Glycan uptake across the bacterial outer membrane (OM) of these bacteria is mediated by SusCD protein complexes, comprising a membrane-embedded barrel and a lipoprotein lid, that is thought to open and close to facilitate substrate binding and transport. Here we show that for both the levan and dextran utilisation systems of Bacteroides thetaiotaomicron, the additional OM components assemble on the core SusCD transporter, forming stable glycan utilising machines which we term ‘utilisomes’. Transport-competent FOS are generated from levan by a surface-exposed lipoprotein, a GH32-family levan endo-glycanase (GHlev), while an SGBP (SGBPlev) is thought to recruit levan at the cell surface. Single particle cryogenic electron microscopy (cryoEM) structures in the absence and presence of substrate reveal concerted conformational changes that demonstrate the mechanism of substrate capture, and rationalise the role of each component in the utilisome.

The density is compatible with ~12 β2,6-linked fructose units in an extended conformation, with a putative β2,1 decoration on Frc-7. Levan binding at this tethering site is also seen in GHlev in the absence of bridging interactions with SGBPlev and in crystal structures of the inactive levanase solved in the presence of FOS of DP ~7-8 (ED Fig. 8). Indeed, secondary binding sites are relatively common in endo-acting GH enzymes, where they may enhance substrate processivity. No ligand was observed at the secondary site in a GHlev structure complexed to a 4 unit FOS (PDB ID 6R3U28), suggesting the affinity for short FOS is low. Single substitution of aromatic residues (to alanine) near the GHlev active site (Y70A and W318A) decreased affinity for levan 25-30 fold, while equivalent substitutions at the tethering site FOS4 had a 6-fold decrease in affinity (W217A) or no effect (F243A and Y437A). These results suggest the active site (FOS3) is responsible for most of the affinity of GHlev for levan. However, numerous weak interactions within the extensive secondary site (FOS4) including polar residues, may result in a substantial overall affinity and specificity.

>[2x]MMKNMILPIAFTALIASMTACSDETDPILTQKNWDGTATYFQSSDEHGFSMYYKPQVGFVGNPMPFYDPVAKDFKVMYLQDYRPNPEATYHPIFGVATKDGATYESLGELISCGGRDEQDAAIGTGGTIYNPADKLYYTFYTGNKFKPSSDQNAQVVMVATSPDFKTWTKNRTFYLKGDTYGYDKNDFRDPFLFQTEDGVYHMLIATRKNGKGHIAEFTSADLKEWESAGTFMTMMWDRFYECPDVFKMGDWWYLIYSEQASFMRKVQYFKGRTLEDLKATTANDAGIWPDNREGMLDSRAFYAGKTASDGTNRYIWGWCPTRAGNDNGNVGDVEPEWAGNLVAQRLIQHEDGTLTLGVPDAIDRKYTSAQEVKVMAKDGNMIESGKTYTLGEGASVIFNRLKVHNKISFTVKTASNTDRFGISFVRGTDSASWYSIHVNADEGKANFEKDGDDAKYLFDNKFNIPADNEYRVTIYSDQSVCVTYINDQLSFTNRIYQMQKNPWSLCCYKGEITVSDVQVSTY[(2~{R},3~{S},4~{R},5~{R})-5-[7-azanyl-5-(hydroxymethyl)benzimidazol-1-yl]-3,4-bis(oxidanyl)oxolan-2-yl]methyl 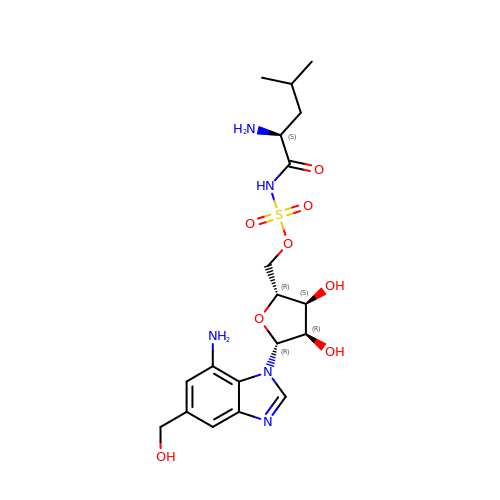~{N}-[(2~{S})-2-azanyl-4-methyl-pentanoyl]sulfamate | C19 H29 N5 O8 S | KLFPFKQOJXUPER-MVGUPFISSA-N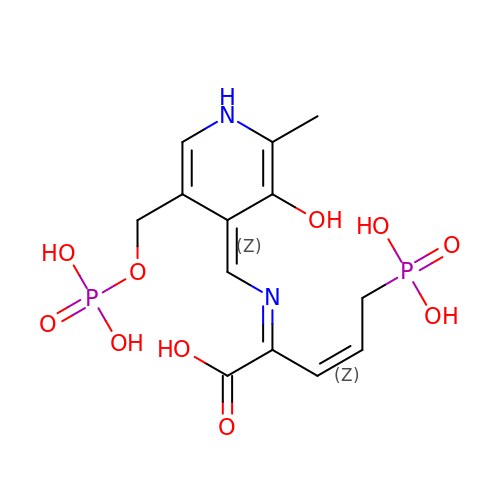(2E,3Z)-2-{[(Z)-{3-hydroxy-2-methyl-5-[(phosphonooxy)methyl]pyridin-4(1H)-ylidene}methyl]imino}-5-phosphonopent-3-enoic acid | C13 H18 N2 O10 P2 | XGSUDZJIHIXLDE-NTUDHWJFSA-N> AKGTTCQKAIVNWEAANPGKNPSEAEEIKLIFQIPPIEKMDGPV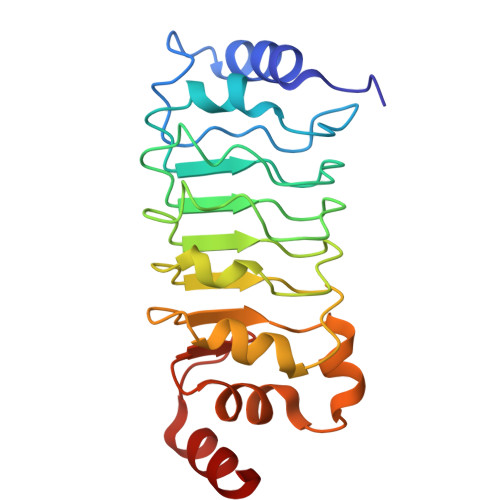LNTLTKCKKLSLSSNSIDKMISLNMLRNLEILSLSRNVIKKISGLEDIGGTLRQLWLSYNFIEKLDGLNNCSVLQTLYIGNNRIKNWEELDKLKDLPELENVLFYGNPIYEQVKEDPKLIVLKKLPTLKNVDGYIIDDSVLEKVKQIA PERINDOPRILAT | C17 H28 N2 O5 | 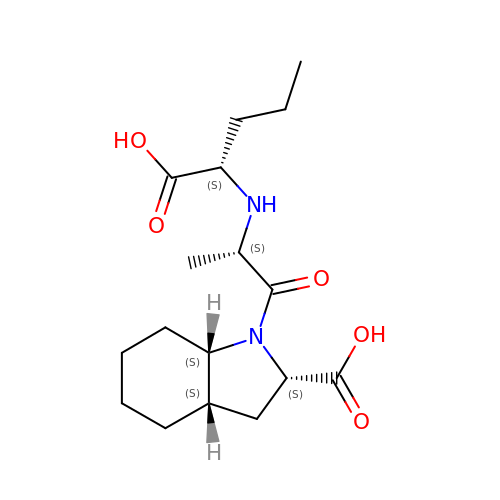ODAIHABQVKJNIY-PEDHHIEDSA-N>MTLYSCCLILLLFTWNTAAYGPNQRAQKKGDIILGGLFPIHFGVAAKDQDLKSRPESVECIRYNFRGFRWLQAMIFAIEEINNSPNLLPNMTLGYRIFDTCNTVSKALEATLSFVAQNKIDSLNLDEFCNCSEHIPSTIAVVGATGSGVSTAVANLLGLFYIPQVSYASSSRLLSNKNQFKSFLRTIPNDEHQATAMADIIEYFRWNWVGTIAADDDYGRPGIEKFREEAEERDICIDFSELISQYSDEEEIQQVVEVIQNSTARVIVVFSSGPDLEPLIKEIVRRNITGKIWLASEAWASSSLIAMPEFFRVIGSTIGFALKAGQIPGFREFLQKVHPKKSANNGFAKEFWEETFNCYLPSESKNSPASASFHKAHEEGLGAGNGTAAFRPPCTGDENITSVETPYMDFTHLRISYNVYLAVYSIAHALQDIYTCTPGKGLFTNGSCADIKKVEAWQVLKHLRHLNFTSNMGEQVDFDEFGDLVGNYSIINWHLSPEDGSVVFEEVGHYNVYAKKGERLFINENKILWSGFSKEVPFSNCSRDCLPGTRKGIIEGEPTCCFECVDCPDGEYSDETDASACDKCPEDYWSNENHTSCIPKQIEFLSWTEPFGIALTLFAVLGIFLTSFVLGVFTKFRNTPIVKATNRELSYLLLFSLLCCFSSSLFFIGEPQNWTCRLRQPAFGISFVLCISCILVKTNRVLLVFEAKIPTSLHRKWWGLNLQFLLVFLCTFVQIVICVIWLYTAPPSSYRNHELEDEIIFITCHEGSLMALGFLIGYTCLLAAICFFFAFKSRKLPENFNEAKFITFSMLIFFIVWISFIPAYASTYGKFVSAVEVIAILAASFGLLACIFFNKVYIILFKPSRNTIEEVRCSTAAHAFKVAARATLRRSNVSRKRSNSLGGSTGSTPSSSISSKSNHEDPFPLPASAERQRQQQRGCKQKVSFGSGTVTLSLSFEEPQKNAMANRNAKRRNSLEAQNSDDSLMRHRALLALQNSESLSAEPGFQTASSPETSSQESVVGDNKEEVPNPEAEPSLPSANSRNFIGTGGSSVTENTVHSLESALEVLFQ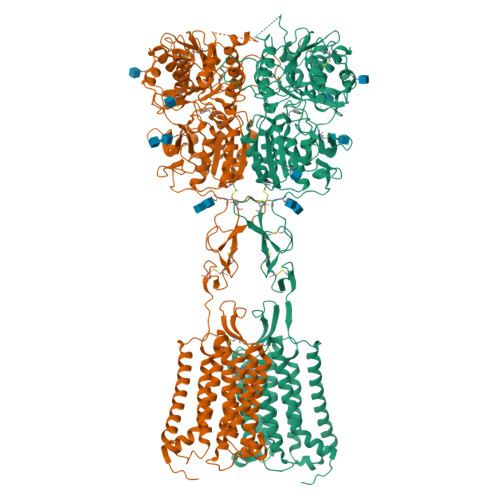[2x]The periplasmic binding protein (PBP) CeuE1 is an important component of the Fe(III) uptake system in Campylobacter jejuni, a commensal Gram-negative bacterium in the avian gut, but a common source of food poisoning in humans. CeuE, an integral part of the CeuBCDE ABC transporter of C. jejuni, is responsible for capturing Fe(III)-siderophore complexes in the periplasm for delivery to their respective inner membrane transporter. C. jejuni does not itself synthesize siderophores, but capitalizes on their secretion by other bacteria, such as E. coli. Here we report a combined solution and structural study of a series of synthetic tetradentate analogues of the enterobactin-derived bis(2, 3-dihydroxybenzoyl-L-Ser), to explore the ligand-binding promiscuity of CeuE, both wild type and with mutations of the Fe(III) binding residues H227 and Y288.

To probe the relative contributions of His227 and Tyr288 to Fe(III)-siderophore binding, site-directed mutagenesis was then used to replace the side chains of the two Fe(III)-coordinating amino acids with non-coordinating side chains of similar size. In addition, the double mutants H227L/Y288F and H227A/Y288F were created. All five mutants (Y288F, H227L, H227A, H227L/Y288F, H227A/Y288F) were crystallized in their apo form, and all structures are closely similar to that of wild type CeuE. However while there is clear electron density for the Y288F mutation in its three structures, H227L and H227A are located in a flexible loop region and there is generally no electron density to confirm their presence. Mutation of the Fe(III)-coordinating tyrosine led to a drastic drop in binding affinity in both the single (Y228F) and the double mutants (H227L/Y288F and H227A/Y288F), with Kd values above 1 μM. Site-directed mutagenesis of CeuE revealed that Y288 is essential for binding, as the binding affinity observed in the fluorescence titration experiments is far weaker for all mutants containing Y228F when compared to the wild type protein. This finding is confirmed by the lack of CD signal corresponding to the Λ-configuration when Fe-5-Lic is added to these mutants.

>[2x]GPAMLPISMSDEGDSFLVKDSLGENKIPKNPSKVVILDLGILDTFDALKLNDKVVGVPAKNLPKYLQQFKNKPSVGGVQQVDFEAINALKPDLIIISGRQSKFYDKLKEIAPTLFVGLDNANFLSSFENNVLSVAKLYGLEKEALEKISDIKNEIEKAKSIVDEDKKALIILTNSNKISAFGPQSRFGIIHDVLGINAVDENIKVGTAGKSINSEFILEKNPDYIFVVDRNVILGNKERAQGILDNALVAKTKAAQNKKIIYLDPEYWFLASGNGLESLKTMILEIKNAVK;> GPAMLPISMSDEGDSFLVKDSIGENKIPKNPSKVVILDLGILDTFDALKLNDKVVGVPAKNLPKYLQQFKNKPSVGGVQQVDFEAINALKPDLIIISGRQSKFYDKLKEIAPTLFVGLDNANFLSSFENNVLSVAKLYGLEKEALEKISDIKNEIEKAKSIVDEDKKALIILTNSNKISAFGPQSRFGIIHDVLGINAVDENIKVGTAGKSINSEFILEKNPDYIFVVDRNVILGNKERAQGILDNALVAKTKAAQNKKIIYLDPEYWFLASGNGLESLKTMILEIKNAVK> GSFTMDHYLDIRLRPDPEFPPAQLMCVLFGKLHQALVAQGGDRIGVSFPDLDESRSRLGERLRIHASADDLRALLARPWLEGLRDHLQFGEPAVVPHPTPYRQVSRVQAKSNPERLRRRLMRRHDLSEEEARKRIPDTVARTLDLPFVTLRSQSTGQHFRLFIRHGPLQVTAEEGGFTC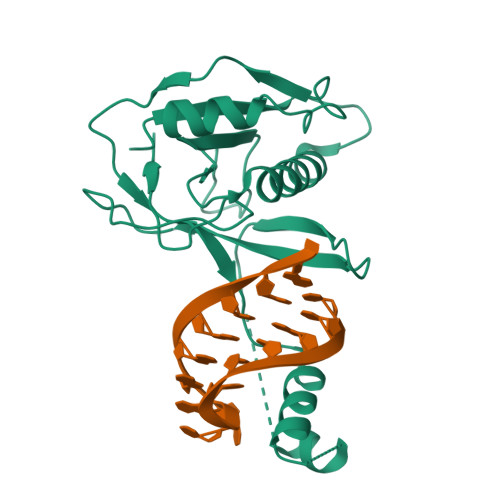YGLSKGGFVPWF> SMKITSSNFATIATSENFAKLSVLPKNHREPIKGLFKSAVEQFSSARDFFKNE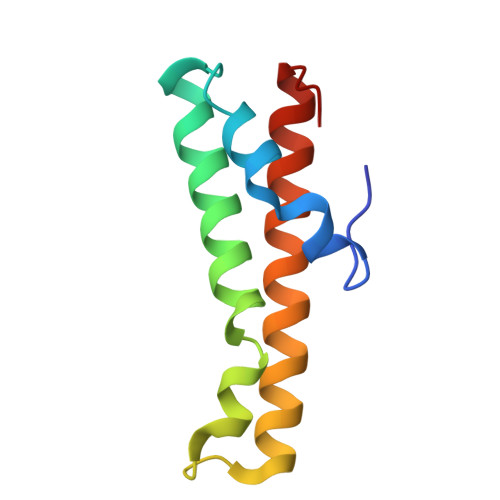NYSKELAEKFNKEAVNEAVEKLQKAIDLAEKQGIQF> MSTAAKQNRSTSRVSKKKTAAPKEGAAKKSDKGHKYEYVELAKASLTSAQPQHFYAVVIDATFPYKTNQERYICSLKIVDPTLYLKQQKGAGDASDYATLVLYAKRFEDLPIIHRAGDIIRVHRATLRLYNGQRQFNANVFYSSSWALFSTDKRSVTQEINNQDAVSDTTPFSFSSKHATIEKNEISILQNLRKWANQYFSSYSVISSDMYTALNKAQAQKGDFDVVAKILQVHELDEYTNELKLKDASGQVFYTLSLKLKFPHVRTGEVVRIRSATYDETSTQKKVLILSHYSNIIT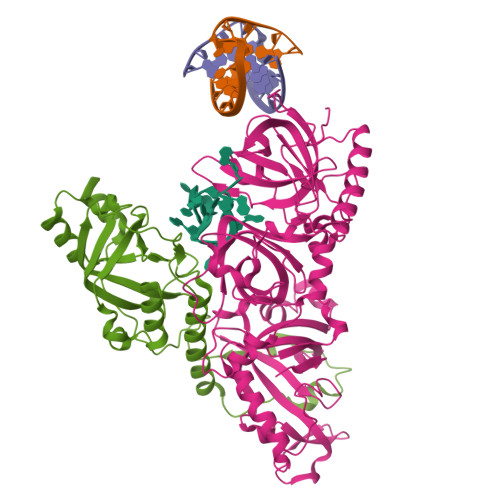FIQSSKLAKELRAKIQDDHSVEVASLKKNVSLNAVVLTEVDKKHAALPSTSLQDLFHHADSDKELQAQDTFRTQFYVTKIEPSDVKEWVKGYDRKTKKSSSLKGASGKGDNIFQVQFLVKDASTQLNNNTYRVLLYTQDGLGANFFNVKADNLHKNADARKKLEDSAELLTKFNSYVDAVVERRNGFYLIKDTKLIY;> MSKGASAPQQQSAFKQLYTELFNNEGDFSKVSSNLKKPLKCYVKESYPHFLVTDGYFFVAPYFTKEAVNEFHAKFPNVNIVDLTDKVIVINNWSLELRRVNSAEVFTSYANLEARLIVHSFKPNLQERLNPTRYPVNLFRDDEFKTTIQHFRHTALQAAINKTVKGDNLVDISKVADAAGKKGKVDAGIVKASASKGDEFSDFSFKEGNTATLKIADIFVQEKGKDALNKAADHTDGAKVKGGAKGKGKAAAKAAKGKKL> FAIDPLKHSKLYEEYGLYLRPHQINQEIKPTTIKKKELAPTIRSIKYASLIHSMLAEHAARHNGTLINPRMYADMITLGNTKVTVTKGTPKAQIDTLKMNGLTVVSKSRRNNKKKPVSDTTATIDENTNAIV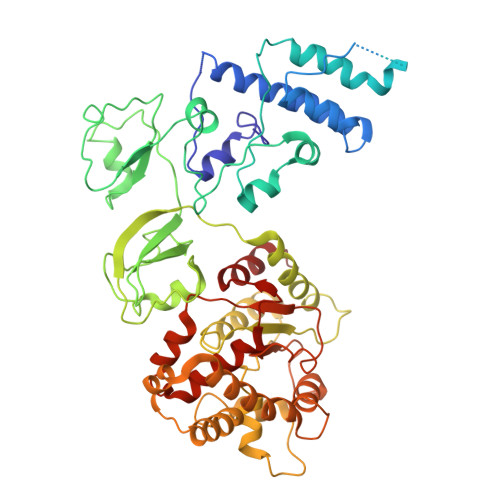TYKALTEMSTLIESFRLPSGLTLIIFDDEKYQSLIPNYINQLIAYTQPHIIPTWQGIADFSDTYLRSYFKRPFELTASNLAAPQKHNLSPMTRSIFNNTGREDAVIRKLYGYGEYVFIKYEGCLITWTGIYGEVTMMVNLSKRDLGLDVGDDYLKEYKKLLFYGVITDAIPSGISTRSTIMKISPHKMMNPSGGALAVLSKFLEAVVSTNVINATLVVYAEKGAGKTSFLSTYAEQLSLASGQVVGHLSSDAYGRWLAKTKDIEEPSFAYDYVLSLDTDDNESYYEQKASELLMSHGISEVAQYELLSVRKKIKMMDEMNEVLIAQLENADTHSERNFYYMVSTGKTTPRILIVEGHFNAQDATIARTDTTVLLRTINDTTQAMRDRQRGGVVQLFLRDTYYRLLPALHTTVYPFEMLESIKRWKWV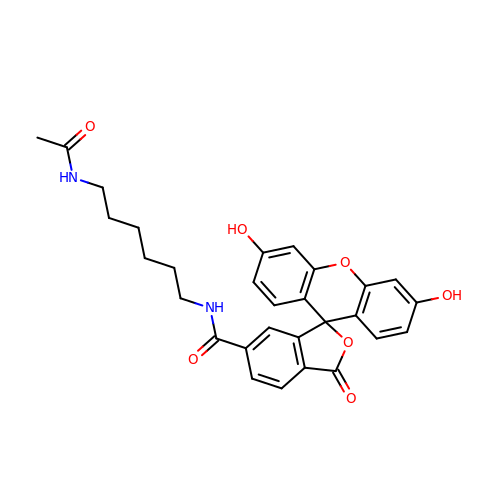N-[6-(ACETYLAMINO)HEXYL]-3',6'-DIHYDROXY-3-OXO-3H-SPIRO[2-BENZOFURAN-1,9'-XANTHENE]-6-CARBOXAMIDE | C29 H28 N2 O7 | NYDPRVGMTFCAQC-UHFFFAOYSA-N> GSDDGAFGDIWAYMSEALTGAPGKIIACGMLFSVAYFGVVKPNLGLALVSALMMLVMANGEKIISSFLDAGIPL

DNA transfer is facilitated by a type IV secretion system (T4SS) nanomachine, embedded in the bacterial cell wall, which is extended by a long hollow filament, known as the conjugation, mating, or sex pilus. Functionally, the pilus is involved in mating pair formation (MPF), linking donors and recipients at a distance. Structures of mating or conjugation pili from the IncF and IncW incompatibility plasmids have revealed that the pilins polymerize into a helical arrangement with tightly bound phospholipid molecules, forming thin, tubular filaments ~8 nanometers in diameter that can extend several micrometers in length. Conjugation pilins are composed of three α helices, α1-3.

Using a derivative of the reference IncHI1 plasmid, R27, a tetracycline resistance plasmid isolated from Salmonella enterica serovar Typhi, we determined the cryo-EM structure of the H-pilus at 2.2 Å resolution. We processed data using standard helical reconstruction in cryoSPARC and reconstructed a map of the H-pilus at 2.2 Å resolution (map:map FSC, 0.143 threshold), by imposing helical (rise 12.14 Å, twist 28.98°) and C5 symmetries. The assembled pilus structure displays an outer diameter of ~ 90 Å and a lumen diameter of ~ 22 Å, which is similar to previously reported conjugation pilus structures. Like other pilins, the TrhA pilin is composed of three α-helices: α1 (Gly8-Thr19), α2 (Ala21-Phe37), and α3 (Gly45-Phe66), connected by short loops. Uniquely, we found that unlike the F and W pilin structures, TrhA is cyclic, formed by a covalent bond connecting the peptide backbone between the N and C termini. The density map unambiguously demonstrated the formation of a peptide bond between Gly1 and Asp69. Although the mature TrhA pilin consists of 74 amino acids, only density for the first 69 residues was visible in the maps, indicating that the five C-terminal residues were cleaved during the cyclization process. The formation of a cyclic structure between N and C termini brings the α1-2 and α3 helical regions closer, likely contributing to the reduced kink angle. In the cyclization region, the main chain atoms of Gly1 and Asp69 participate in a hydrogen bonding network involving Lys24 and ordered water molecules, further stabilizing their structure. Our analysis revealed clear phospholipid density in the map, indicating a precise 1:1 stoichiometry between pilus subunits and phospholipids.>[12x]MTVAKAIFIKCGNLGTSMMMDMLLDERADREDVEFRVVGTSVKMDPECVEAAVEMALDIAEDFEPDFIVYGGPNPAAPGPSKAREMLADSEYPAVIIGDAPGLKVKDEMEEQGLGYILVKPDAMLGARREFLDPVEMAIYNADLMKVLAATGVFRVVQEAFDELIEKAKEDEISENDLPKLVIDRNTLLEREEFENPYAMVKAMAALEIAENVADVSVEGCFVEQDKERYVPI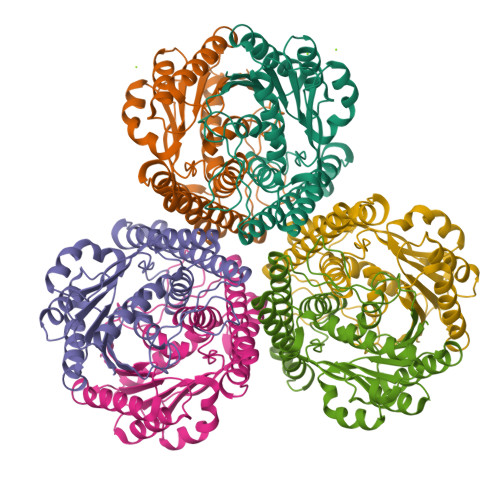VASAHEMMRKAAELADEARELEKSNDAVLRTPHAPDGKVLSKRKFMEDPE> MGSSHHHHHHGSNQLTAYTLRLGDNCLVLSQRLGEWCGHAPELEIDLALANIGLDLLGQARNFLSYAAELAGEGDEDTLAFTRDERQFSNLLLVEQPNGNFADTIARQYFIDAWHVALFTRLM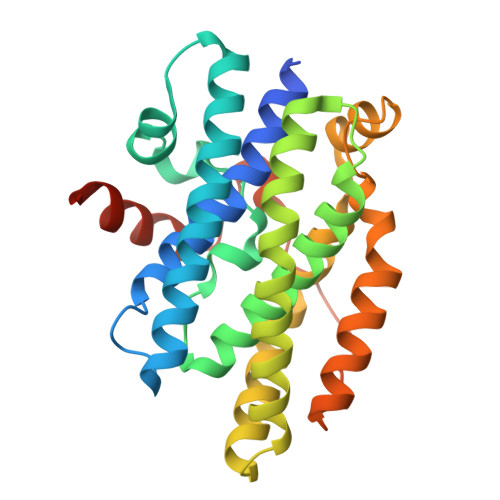ESRDPQLAAISAKAIKEARYHLRFSRGWLERLGNGTDVSGQKMQQAINKLWRFTAELFDADEIDIALSEEGIAVDPRTLRAAWEAEVFAGINEATLNVPQEQAYRTGGKKGLHTEHLGPMLAEMQYLQRVLPGQQW> ASAPIGSAISRNNWAVTCDSAQSGNECNKAIDGNKDTFWHTFYGANGDPKPPHTYTIDMKTTQNVNGLSMLPRQDGNQNGWIGRHEVYLSSDGTNWGSPVASGSWFADSTTKYSNFETRPARYVRLVAITEANGQPWTSIAEINVFQASSYTAPQPGLGRWGPTIDLPIVPAAAAIEPTSGRVLMWSSYRNDAFGGSPGGITLTSSWDPSTGIVSDRTVTVTKHDMFCPGISMDGNGQIVVTGGNDAKKTSLYDSSSDSWIPGPDMQVARGYQSSATMSDGRVFTIGGSWSGGVFEKNGEVYSPSSK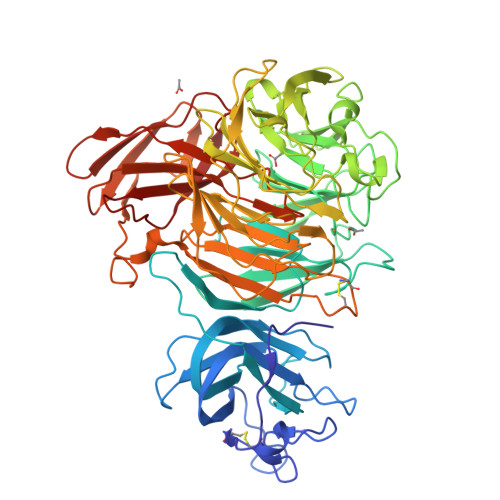TWTSLPNAKVNPMLTADKQGLYRSDNHAWLFGWKKGSVFQAGPSTAMNWYYTSGSGDVKSAGKRQSNRGVAPDAMSGNAVMYDAVKGKILTFGGSPDYQDSDATTNAHIITLGEPGTSPNTVFASNGLYFARTFHTSVVLPDGSTFITGGQRRGIPFEDSTPVFTPEIYVPEQDTFYKQNPNSIVRVYHSISLLLPDGRVFNGGGGLCGDCTTNHFDAQIFTPNYLYNSNGNLATRPKITRTSTQSVKVGGRITISTDSSISKASLIRYGTATHTVNTDQRRIPLTLTNNGGNSYSFQVPSDSGVALPGYWMLFVMNSAGVPSVASTIRVTQ> GSHMAALRERAGPVTWVMMIACVVVFIAMQILGDQEVMLWLAWPFDPTLKFEFWRYFTHALMHFSLMHILFNLLWWWYLGGAVEKRLGSGKLIVITLISALLSGYVQQKFSGPWFGGLSGVVYALMGYVWLRGERDPQSGIYLQRGLIIFALIWIVAGWFDLFGMSMANGA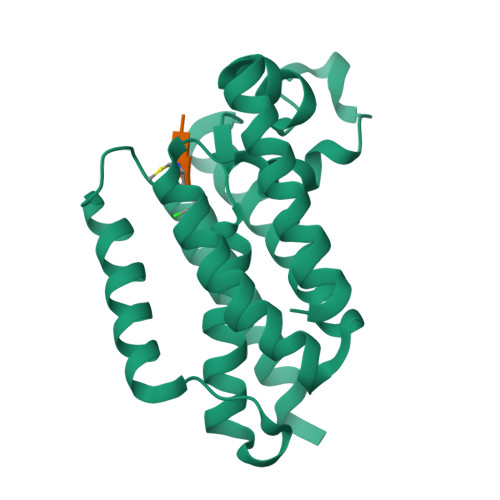HIAGLAVGLAMAFVDSLNARKRK> TSWSDRLQNAADMPANMDKHALKKYRREAYHRVFVNQSLAMEKIKCFGFDMDYTLAVYKSPEYESLGFELTVERLVSIGYPQELLSFAYDSTFPTRGLVFDTLYGNLLKVDAYGNLLVCAHGFNFIRGPETREQYPNKFIQRDDTERFYILNTLFNLPETYLLACLVDFFTNCPRYTSCETGFKDGDLFMSYRSMFQDVRDAVDWVHYKGSLKEKTVENLEKYVVKDGKLPLLLSRMKEVGKVFLATNSDYKYTDKIMTYLFDFPHGPKPGSSHRPWQSYFDLILVDARKPLFFGEGTVLRQVDTKTGKLKIGTYTGPLQHGIVYSGGSSDTICDLLGAKGKDILYIGDHIFGDILKSKKRQGWRTFLVIPELAQELHVWTDKSSLFEE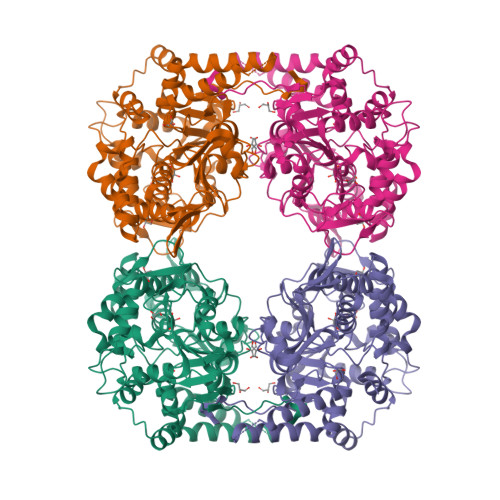LQSLDIFLAELYKHLDSSSIQRRIKKVTHDMDMCYGMMGSLFRSGSRQTLFASQVMRYADLYAASFINLLYYPFSYLFRAAHVLMPHES>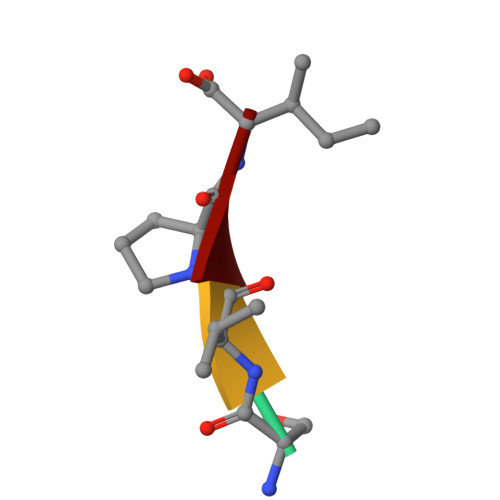 SVPI> GSSPSLEQDDGDEETSVVIVGKISFCPKDVLGHGAEGTIVYRGMFDNRDVAVKRILPECFSFADREVQLLRESDEHPNVIRYFCTEKDRQFQYIAIELCAATLQEYVEQKDFAHLGLEPITLLQQTTSGLAHLHSLNIVHRDLKPHNILISMPNAHGKIKAMISDFGLCKKLAVGRHSFSRRSGVPGTEGWIAPEMLSEDCKENPTYTVDIFSAGCVFYYVISEGSHPFGKSLQRQANILLGACSLDCLHPEKHEDVIARELIEKMIAMDPQKRPSAKHVLKHPFFWSLEKQLQFFQDVSDRIEKESLDGPIVKQLERGGRAVVKMDWRENITVPLQTDLRKFRTYKGGSVRDLLRAMRNKKHHYRELPAEVRETLGSLPDDFVCYFTSRFPHLLAHTYRAMELCSHERLFQPYYFHEPPEPQPPVTPDALGNS

IRE1 integrates multiple functional domains into a single ER-membrane-spanning protein. The lumenal domain senses unfolded proteins in the ER through indirect and direct mechanisms: as a result, it undergoes dimerization and subsequent oligomerization. The association of the lumenal domain promotes dimerization and oligomerization of the cytoplasmic kinase-RNase tandem domain. The cytoplasmic domain has been shown to self-associate via different surface contacts, where a back-to-back (B2B) configuration is believed to fulfill the essential structural requirements for RNase activation.

We determined the crystal structures of G-9807 and G-1749 in complex with IRE1-0P at about 2 Å resolution. The structures are shown in Fig. 2 together with the structures of AMG-18-bound-31 and apo IRE1, including the first reported crystal structure of human apo IRE1-3P. All structures show IRE1 as a B2B dimer, with extensive overlay of the RNase domains, but some differences in the kinase domains, especially in the conformation of the activation loop and αEF-αF loop. In IRE1 apo structures and IRE1 in complex with allosteric activators, D620 and E621 of one monomer form salt bridges with R627 and K706, respectively, of the second monomer, while in the AMG-18 structure D620 has flipped outward due to the helix unwinding, hindering hydrogen bond formation with K706 and interacting instead with the backbone of A701. IRE1-0P was predominantly monomeric up to a concentration of 30 µM, while phosphorylation partially stabilized the IRE1 dimer as expected, with a calculated dimerization Kd = 67 µM.> SNAMTIATIDIGGTGIKFASLTPDGKILDKTSISTPENLEDLLAWLDQRLSEQDYSGIAMSVPGAVNQETGVIDGFSAVPYIHGFSWYEALSSYQLPVHLENDANCVGLSELLAHPELENAACVVIGTGIGGAMIINGRLHRGRHGLGGEFGYMTTLAPAEKLNNWSQLASTGNMVRYVIEKSGHTDWDGR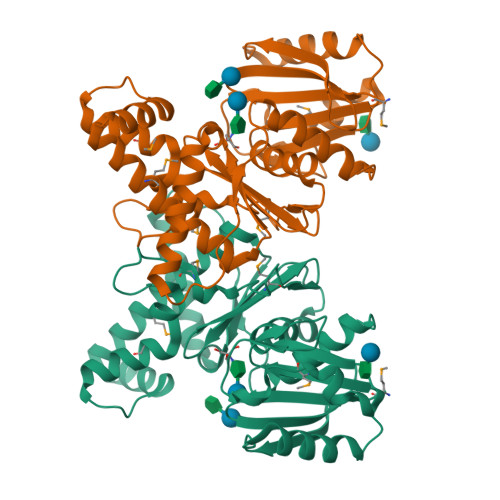KIYQEAAAGNILCQEAIERMNRNLAQGLLNIQYLIDPGVISLGGSISQNPDFIQGVKKAVEDFVDAYEEYTVAPVIQACTYHADANLYGALVNWLQEEKQW> MVTVVEEVDHLPIYDLDPKLEEFKDHFNYRIKRYLDQKCLIEKHEGGLEEFSKGYLKFGINTVDGATIYREWAPAAQEAQLIGEFNNWNGAKHKMEKDKFGIWSIKISHVNGKPAIPHNSKVKFRFRHGGGAWVDRIPAWIRYATFDASKFGAPYDGVHWDPPACERYVFKHPRPPKPDAPRIYEAHVGMSGEEPEVSTYREFADNVLPRIRANNYNTVQLMAIMEHSYYASFGYHVTNFFAVSSRSGTPEDLKYLVDKAHSLGLRVLMDVVHSHASNNVTDGLNGYDVGQNTHESYFHTGDRGYHKLWDSRLFNYANWEVLRFLLSNLRYWMDEFMFDGFRFDGVTSMLYHHHGINKGFTGNYKEYFSLDTDVDAIVYMMLANHLMHKLLPEATIVAEDVSGMPVLCRPVDEGGVGFDFRLAMAIPDRWIDYLKNKEDRKWSMSEIVQTLTNRRYTEKCIAYAESHDQSIVGDKTIAFLLMDKEMYTGMSDLQPASPTINRGIALQKMIHFITMALGGDGYLNFMGNEFG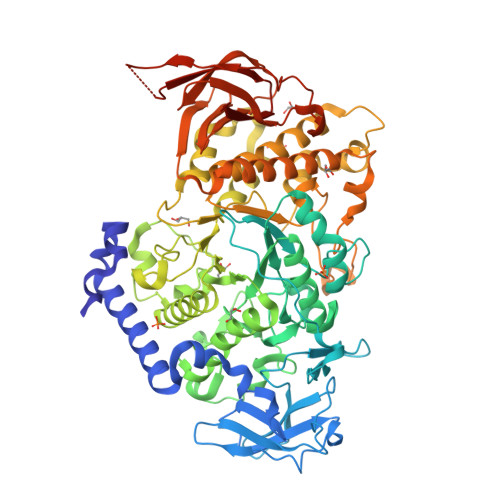HPEWIDFPREGNNWSYDKCRRQWSLVDTDHLRYKYMNAFDQAMNALEEEFSFLSSSKQIVSDMNEKDKVIVFERGDLVFVFNFHPNKTYKGYKVGCDLPGKYRVALDSDALVFGGHGRVGHDVDHFTSPEGMPGVPETNFNNRPNSFKVLSPPRTCVAYYRVDEDREELRR Here, we report the crystal structure of hAQP10, the only human aquaglyceroporin that becomes stimulated by pH reduction, in agreement with the altered cellular conditions observed during lipolysis in human adipocytes. In contrast to other known aquaporin structures, hAQP10 displays pH-dependent glycerol-specific gating at the intracellular interface, rather than flux governed by the classical selectivity filter. Specifically, we identify H80 as a critical part for this regulation, being the pH-sensor that propagates structural rearrangements leading to the opening of hAQP10, upon double protonation associated with low pH conditions. Our combined analyses reveal that pH regulation is achieved by a cytoplasmic, glycerol-specific gate and, likely, a widened ar/R filter, both unique to hAQP10, correlating with intracellular acidification of adipocytes observed during lipolysis.

However, full-length hAQP10 yielded no crystals and we continued with a variant (hAQP10cryst) truncated in the termini (Δ1–10, Δ278–301) that crystallized at pH 6.0. The structure was determined at 2.3 Å resolution, and reveals a tetramer fold highly reminiscent of other AQPs, with each monomer formed by six transmembrane helices (TM1–TM6) establishing a conducting channel. Strikingly, the region typically linked to selectivity in AQPs, the aromatic and arginine (ar/R) selectivity filter at the non-cytosolic end of the pore, is significantly wider (2.6 Å) than in previously structurally characterized AQPs, as also found by HOLE analyses. A single glycerol molecule is instead located adjacent to the AQP archetypical, central NPA-motif (N82–A84) in hAQP10. However, toward the cytoplasm the glycerol molecule is rather positioned close to the unique F85 of loop B in hAQP10 (invariant as a valine/isoleucine in other AQPs). F85 has a side-chain configuration unfavorable for glycerol passage, forming a unique mechanistic feature. Moreover, the entire cytoplasmic pore region has adapted a tight arrangement not previously observed, achieved by the first part of loop B (G73-H80; loop layout likely allowed by the hAQP10-specific G73G74-motif) with V76-S77 capping the cytoplasmic opening, F85, and R94 (of TM3), which seemingly stabilizes loop B in the closed configuration. Notably, HOLE analysis suggests that this narrowing (0.9 Å) permits water (0.8 Å at the ar/R filter in hAQP2), but not glycerol (1.3 Å in AqpM)16 flux, in agreement with the proteopolymersome data at relatively high pH. Nevertheless, as the obtained crystal form contains the entire hAQP10 tetramer in the asymmetric unit, intermonomeric differences were analyzed. While overall highly similar, three chains (Fig. 2b dark gray and Supplementary Fig. 7c) display an identical, closed, cytoplasmic arrangement.

>[4x]MVFTQAPAEIMGHLRIRSLLARQCLAEFLGVFVLMLLTQGAVAQAVTSGETKGNFFTMFLAGSLAVTIAIYVGGNVSGAHLNPAFSLAMCIVGRLPWVKLPIYILVQLLSAFCASGATYVLYHDALQNYTGGNLTVTGPKETASIFATYPAPYLSLNNGFLDQVLGTGMLIVGLLAILDRRNKGVPAGLEPVVVGMLILALGLSMGANCGIPLNPARDLGPRLFTYVAGWGPEVFSAGNGWWWVPVVAPLVGATVGTATYQLLVALHHPEGPEPAQDLVSAQHKASELETPASAQMLECKL Here, we characterize an upstream component of parasite GPI anchor biosynthesis, the putative phosphomannomutase (PMM) (EC 5.4.2.8), HAD5 (PF3D7_1017400). PMMs are responsible for the conversion of mannose 6-phosphate (M6P) to mannose 1-phosphate (M1P), the precursor to GDP-mannose. HAD5 and other PMMs are part of the haloacid dehalogenase (HAD) superfamily of proteins (Interpro: IPR023214), a ubiquitous family of enzymes that primarily conduct phosphatase and phosphotransferase reactions. By regulating the expression of HAD5 in transgenic parasites with a TetR-DOZI-inducible knockdown system, we demonstrated that HAD5 is required for malaria parasite egress and erythrocyte reinvasion, and we assessed the role of HAD5 in GPI anchor synthesis by autoradiography of radiolabeled glucosamine and thin layer chromatography.

To uncover the structural basis for HAD5-specific inhibition, we solved the X-ray crystal structure of HAD5 to 3.5 Å resolution. Like other known PMMs and members of the HAD superfamily, HAD5 comprises two domains with an overall fold similar to that of HsPMM1. There were no large structural differences in the overall three-dimensional folds of the human and parasite enzymes. Although many active site features between the Plasmodium and human enzymes are conserved, an active site loop contains significant sequence variations. This loop in HAD5 contains Met173, Gln176, and Ile179, whereas the corresponding residues in PMM1 are Arg183, Met186, and Phe189. To develop a model for how compound D9 may interact with HAD5, we computationally docked the ligand into the active site of the HAD5 X-ray crystal structure. The resulting position of D9 in the HAD5 active site is similar to the crystallographically determined binding mode of mannose-1-phosphate in the X-ray structure of human PMM1 (76). The docking solution orients the hydroxyaminomethyl group of compound D9 in proximity to the sidechains of residues in the variable active site loop. Furthermore, comparison of D9 to similar but less potent compounds used for HAD5 inhibitor screening, D7 and D11, indicates that the hydroxyaminomethyl group is a key determinant of HAD5 inhibition compared to the human PMM. Finally, the crystal structure of HAD5 is likely to be valuable to ongoing efforts to develop more potent and specific HAD5 inhibitors as antimalarials.

>GSHMNKKKAIFLFDVDGTLTISRKTIEQNVVDTLLELKSKKGFVLGIVGGSDYKKIREQIKYPEIFDYIFSENGVVAHKNDEEYFAESIVNFLGEDRLKKLINYSLKYIANLDIPKKRGTFIELRNGIINISPIGRNCSQEERDEFFRYNLKNNTIEKFRDNLSKEFEDFDLNFSMGGQISIDCFPKGWDKTFCLKHLENKFDEIYFFGDRTDKGGNDYELFCDKRVKGYKVKNPNDTVKILRENFL[2x]>SELRHLRLPTYQELEQEINTLKADNDALKIQLKYAQKKIESLQL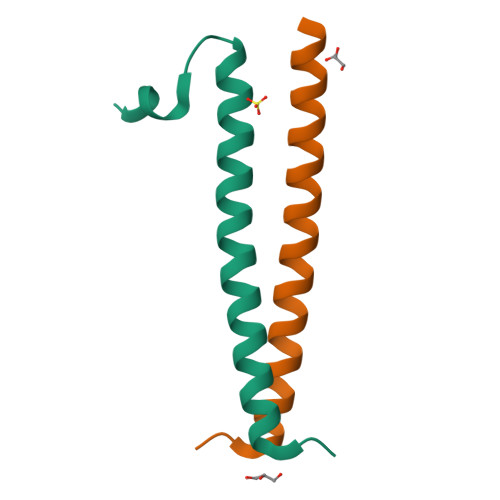EKSNHVLAQMEQ[2x]> MGHHHHHHKQGRLRLAVITTAKYFIPRLLGEFIQKYPGIEVSLKVTNHEQIRHRMQNNEDDLYIVSEPPEEIDLNYQPFLDNPLVVIARRDHPLAGKSNIPITALNDEAFIMREKGSGTRLAVQNLFHRHYVDVRVRLELGSNEAIKQAIAGGMGISVLSQHTLVSEGARSELTILDIDEFPIKRRWYVANLAGKQLSVIT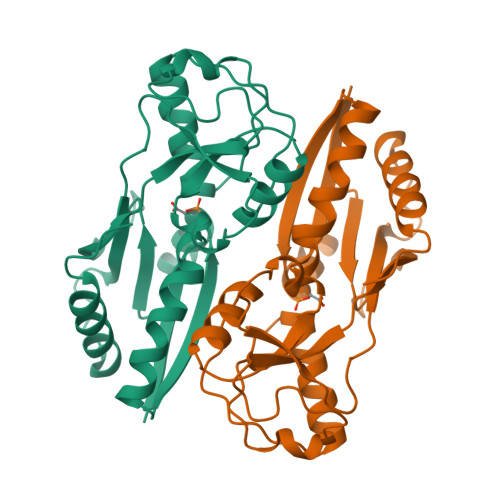QTFLDYLMAVTKNMPAPFAEQLTTQQTPVKLVL> MSDLVWSRDGLDWPHREASRFIEAGGFRWHVQRMGSPAAPAILLIHGTGAASHSWRGLAPLLSRHYHVVAPDLPGHGFTQTPRGHRMSLPGMASDLAALLRVLQVAPQLVV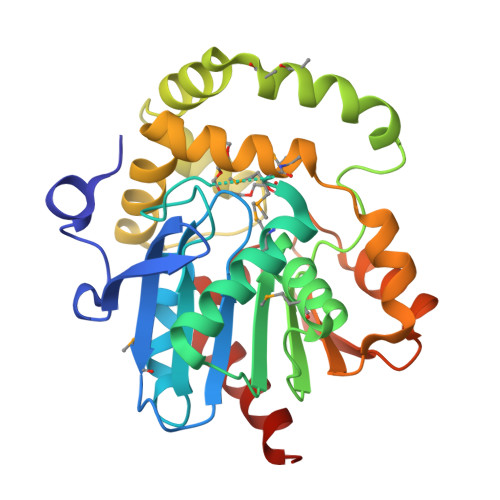GHSAGAAILARMCLDGSIDPKILFSLNGAFLPYGGPAASFFSPLAKMLVMNPFVPSLFAWQAGHRGAVERLIGNTGSTIDPAGIKLYGKLVSSPNHVAAALRMMANWDLEPLLKALPNLKPLLVLVAAEGDRAIPPSVAVKVREILPKAVIERIPALGHLAHEERPALIAALIERYAEKLENIE> MGSSHHHHHHSSGLVPRGSHMASNSTYAPNVDSTVSLKGTDVFKADSASIAQNYTIPEWFKDAKFGIFIHWGVYSVPAYGSEWYSRWMYKEGHPINKYHVQTYGPLTKFGYKDFIPMFKAENFNADEWLAVVKSSGAQYIVPVAEHHDGFAMYSSTFNKWNAVDMGPKRDIIGELKEATKKAGLRFGLSSHRCENAWFYEYGMETPSDVQDTTITLYGERLHEPEGQGMTPYCGKYEGSNERSRRQFLMHTYELIDKYQPELIWFDWTVGKYPFQPTFYKFMAYYYNSALDWNKEVVVNTKFGYGDNIQVFDIERGKSDRIREYPWQTDTSVGKKSWSYCVGEENKSPDHIIDDFVDIVSKNGNLLLNIGPKADGTITD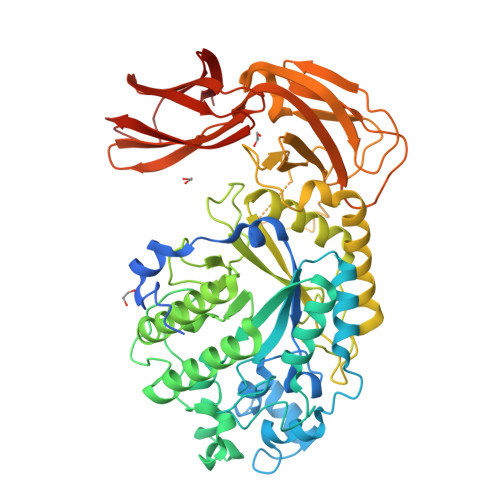EQKNVLAEIGKWLKTNGEAIYGSRPWVIASEGHNAGTAGYMTDNTKTEYTADDIRFTTCDNNLYAVSLAWTDGSVTIKSLATKYCRNVEIESVEMLGSSEKIDYKMTDEGLVVNFPKNKPTEYAHVFKIKLKGVVVSKPLYDKVDNGCLITVRVANHNAEDANVTLKSVVDGNEVSTQVAVKAKSEQWVKMQNKDVKSFDDMSCKFYFNDNLTYENEFKK> MHHHHHHSSGRENLYFQGHMQKLFDTCKKVFADGKSGTVPSQENIEMLRAVLDEIKPEDVGVNPKMSYFRSTVTGRS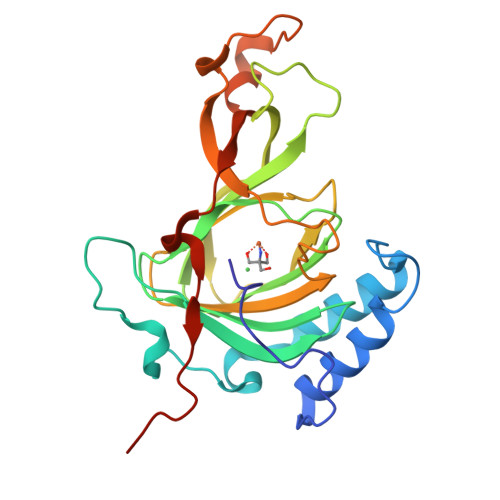PLVTYLHIYACHRFSICIFCLPPSGVIPLHNHPEMTVFSKLLFGTMHIKSYDWVPDSPQPSSDTRLAKVKVDSDFTAPCDTSILYPADGGNMHCFTAKTACAVLDVIGPPYSDPAGRHCTYYFDYPFSSFSVDGVVVAEEEKEGYAWLKEREEKPEDLTVTALMYSGPTIKE>[14x]MNLIPTVIETTNRGERAYDIYSRLLKDRIIMLGSQIDDNVANSIVSQLLFLQAQDSEKDIYLYINSPGGSVTAGFAIYDTIQHIKPDVQTICIGMAASM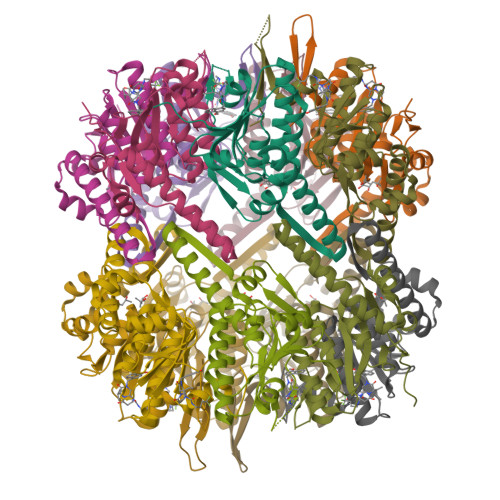GSFLLAAGAKGKRFALPNAEVMIHQPLGGAQGQATEIEIAANHILKTREKLNRILSERTGQSIEKIQKDTDRDNFLTAEEAKEYGLIDEVMVPETKHHHHHH>LPRETDEEPEEPGKKGSFVEMVDNLRGKSGQGYYVEMTVGSPPQTLNILVDTGSSNFAVGAAPHPFLHRYYQRQLSSTYRDLRKGVYVPYTQGKWEGELGTDLVSIPHGPNVTVRANIAAITESDKFFINGSNWEGILGLAYAEIARPDDSLEPFFDSLVKQTHVPNLFSLQLCGAGFPLNQSEVLASVGGSMIIGGIDHSLYTGSLWYTPIRREWYYEVIIVRVEINGQDLKMDCKEYNYDKSIVDSGTTNLRLPKKVFEAAVKSIKAASSTEKFPDGFWLGEQLVCWQAGTTPWNIF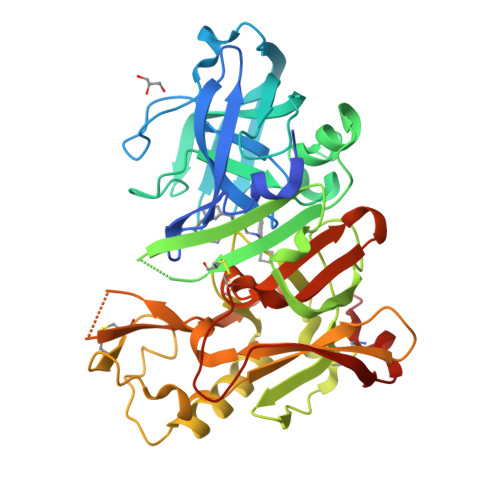PVISLYLMGEVTNQSFRITILPQQYLRPVEDVATSQDDCYKFAISQSSTGTVMGAVIMEGFYVVFDRARKRIGFAVSACHVHDEFRTAAVEGPFVTLDMEDCGYNIPQTDES[3x]dimethyl (1S,2S,4S,5S)-4,5-dihydroxycyclohexane-1,2-dicarboxylate | C10 H16 O6 | 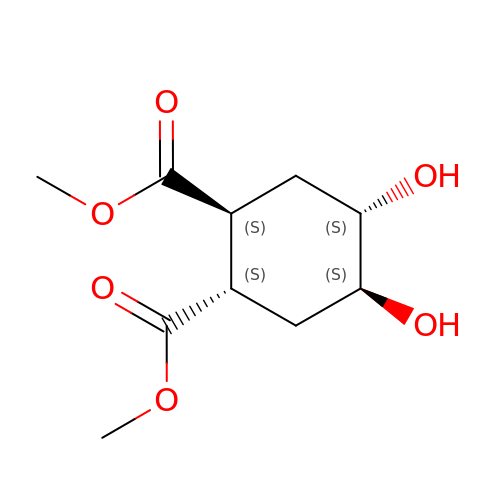ICVNZKRWDVXSLF-XAMCCFCMSA-N>GPLGSPSTLANYYENLVKVFFVSGDPLLHTTAWKKFYKLYSTNPRATEEEFKTYSSTIFLSAISTQLDEIPSIGYDPHLRMYRLLNLDAKPTRKEMLQSIIEDESIYGKVDEELKELYDIIEVNFDVDTVKQQLENLLVKLSSKTYFSQYIAPLRDVIMRRVFVAASQKFTTVSQSELYKLATLPAPLDLSAWDIEKSLLQAAVEDYVSITIDHESAKVTFAKD[2x]

The PCI domain is a conserved bipartite domain comprising the helical bundle (HB) and winged-helix (WH) subdomains initially identified as the principal scaffold for the multisubunit 26S proteasome lid, signalosome (CSN) and eIF3 complexes. Yeast eIF3 contains two PCI domains, one at the N-terminus of its eIF3a/TIF32 subunit and the other at the C-terminus of eIF3c/NIP1. PCI domains are known to be protein interaction sites. a/TIF32, the largest subunit of yeast eIF3, has been implicated in building the core of eIF3 by interacting with c/NIP1 and b/PRT1, two other large eIF3 subunits. Taken together, we propose that one of the key roles of the a/TIF32-PCI domain is, besides building the eIF3 core, to contact mRNAs in a non-specific manner and promote their delivery to and/or stable binding on the small ribosomal subunit.

The crystal structure of a/TIF32276-494 was solved by single wavelength anomalous dispersion using a selenomethionine (SeMet) derivative and refined to the final resolution of 2.65 Å. The asymmetric unit (AU) is composed of two molecules of a/TIF32276−494, which corresponds to a solvent content of 45%. Although the first molecule in the AU (chain A in the pdb file) is almost complete, the second molecule is only partially defined in the electron density map. The crystal structure of a/TIF32276–494 consists of two intimately connected subdomains; an N-terminal right-handed helical bundle capped by a C-terminal winged helix (WH) domain. The helical bundle (HB) is composed of three pairs of antiparallel helices with structural resemblance to tetratricopeptide repeats (TPR). Interestingly, residues 337–362, which form the loop and the helix connecting helices 3 and 4, are not present in the structure of any of the known PCI domains. The winged helix sub-domain shows the canonical α-β-α-α-β-β topology with an N-terminal elongated helix, which is kinked at the beginning. Most notably, R431 of helix 7, E392 of helix 5 and R363 of helix 4 are tightly linked by hydrogen bonds locking these three helices in place. R363 and the adjacent K364 together with R431 contribute to a positively charged surface on the concave face of the protein, proposing a function for this region in mRNA recruitment (see below). The results indicated the formation of a complex with the stoichiometric ratio of nearly 1 (0.944), the dissociation constant (Kd) of 158 nM and a relatively large enthalpy change of −10.23 kcal/mol.>HHHHHHMLEAKFEEASLFKRIIDGFKDYVQLVNF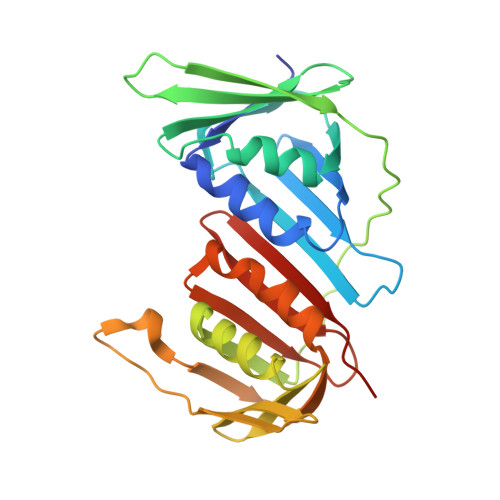QCKEDGIIAQAVDDSRVLLVSLEIGVEAFQEYRCDHPVTLGMDLTSLSKILRCGNNTDTLTLIADNTPDSIILLFEDTKKDRIAEYSLKLMDIDADFLKIEELQYDSTLSLPSSEFSKIVRDLSQLSDSINIMITKETIKFVADGDIGSGSVIIKPFVDMEHPETSIKLEMDQPVDLTFGAKYLLDIIKGSSLSDRVGIRLSSEAPALFQFDLKSGFLQFFLAPKFNDEE[3x]> MGFGELKEEWRGEVVHLSWSPRAFLLKNFLSDEECDYIVEKARPKMVKSSVVDNESGKSVDSEIRTSTGTWFAKGEDSVISKIEKRVAQVTMIPLENHEGLQVLHYHDGQKYEPHYDYFHDPVNAGPEHGGQRVVT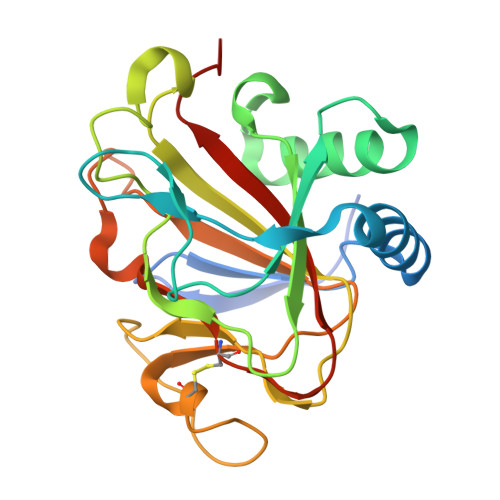MLMYLTTVEEGGETVLPNAEQKVTGDGWSECAKRGLAVKPIKGDALMFYSLKPDGSNDPASLHGSCPTLKGDKWSATKWIHVAPIGGRH(1~{S},4~{R})-3-azabicyclo[2.2.1]hept-5-en-2-one | C6 H7 N O 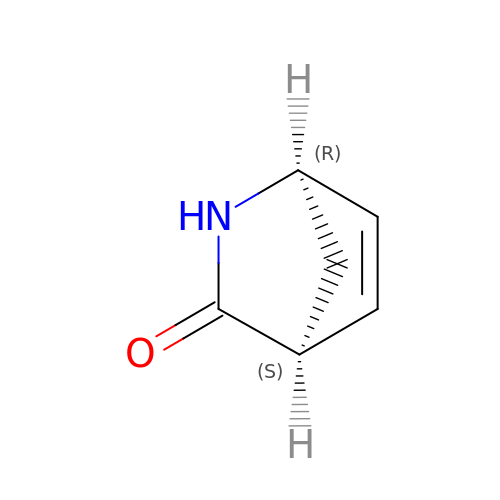| DDUFYKNOXPZZIW-UHNVWZDZSA-N> DVGDEYEIIETIGNGAYGVVSSARRRL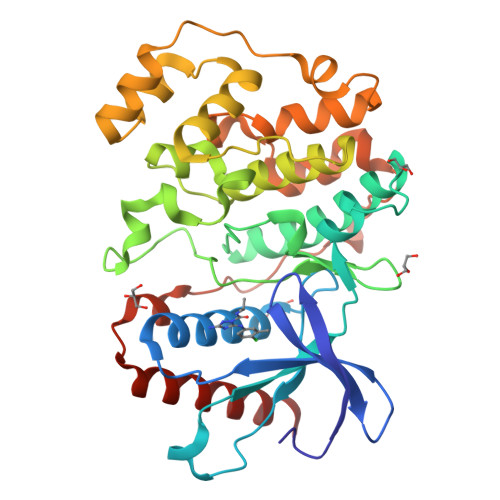TGQQVAIKKIPNAFDVVTNAKRTLRELKILKHFKHDNIIAIKDILRPTVPYGEFKSVYVVLDLMESDLHQIIHSSQPLTLEHVRYFLYQLLRGLKYMHSAQVIHRDLKPSNLLVNENCELKIGDFGMARGLCTSPAEHQYFMTEYVATRWYRAPELMLSLHEYTQAIDLWSVGCIFGEMLARRQLFPGKNYVHQLQLIMMVLGTPSPAVIQAVGAERVRAYIQSLPPRQPVPWETVYPGADRQALSLLGRMLRFEPSARISAAAALRHPFLAKYHDPDDEPDCAPPFDFAFDREALTRERIKEAIVAEIEDFHARRE> PEATSCETEGSSISFTVE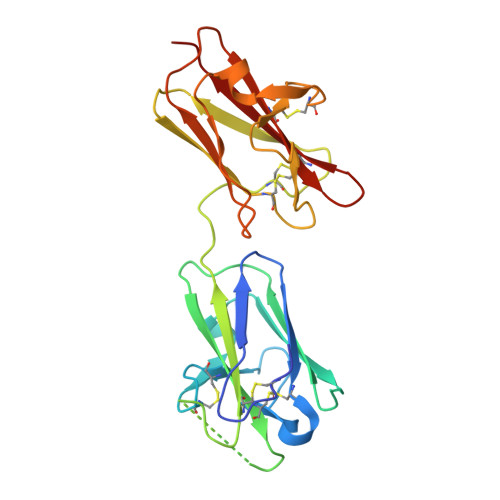KAGHVVRFNCPSTLEEIKPAYEAGDSTKVCTTADCSNEAALKDVLKSASLAQAEGSGPSGGNDFTLTVDALPEAETSVFFLCQRTGASRSARRLGTAVPSDKCGVHILVKAAPQAPVCSAQDHTLELQITAANSDTSFVCGGTFNVIKPANAAKVLQGDSCETEVDLVSLVPHASRSALEQSGLIKLSVTDLPQQQQKLCYRCEDSSQKACKVLVTVSAS>[2x]MRVLLIHSDYIEYEVKDKALKNPEPISEDMKRGRMEEVLVAFISVE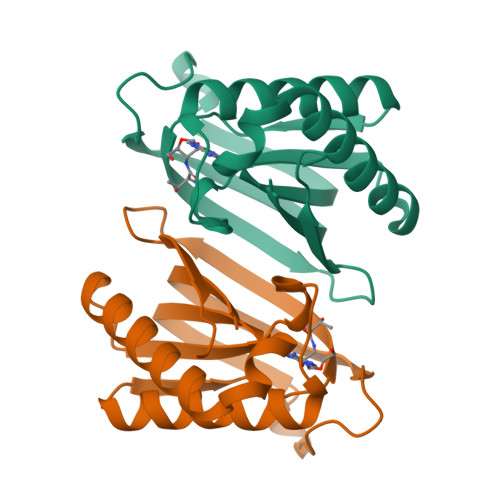KVDEKNPEEVSLKAIEEISKVAEQVKAENVFVYPFAHLSSELAKPSVAMDILNRVYQGLKERGFNVGKAPFGYYMAFKISCKGHPLAELSRTIVPEEARVE> M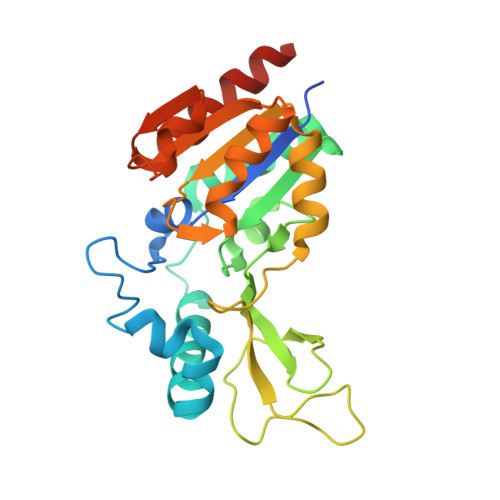GSSHHHHHHSQDPKPRVLVLTGAGISAESGIRTFRAADGLWEEHRVEDVGTPEGFDRDPELVQAFYNARRRQLQQPEIQPNAAHLALAKLQDALGDRFLLVTQNCDNLHERAGNTNVIHMHGELLKVRCSQSGQALDWTGDVTPEDKCHCCQFPAPLRPHVVWFGEMPLGMDEIYMALSMADIFIAIGTSGHVYPAAGFVHEAKLHGAHTVELNLEPSQVGNEFAEKYYGPASQVVPEFVEKLLKGLKAGSIA>AAEKGFKQAFWQPLCQVSEELDDQPKGALFTLQAAASKIQKMRD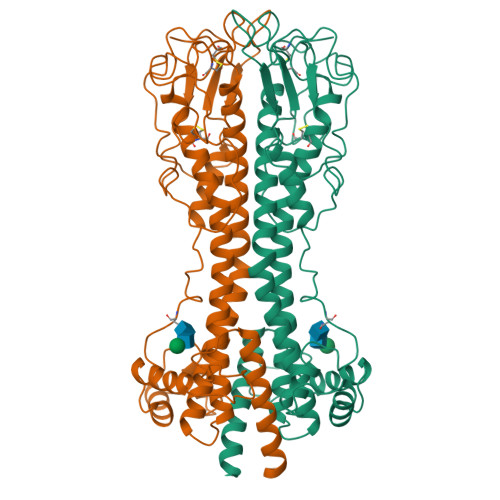AALRASIYAEINHGTNRAKAAVIVANHYAMKADSGLEALKQTLSSQEVTATATASYLKGRIDEYLNLLLQTKESGTSGCMMDTSGTNTVTKAGGTIGGVPCKLQLSPIQPKRPAATYLGKAGYVGLTRQADAANNFHDNDAECRLASGHNTNGLGKSGQLSAAVTMAAGYVTVANSQTAVTVQALDALQEASGAAHQPWIDAWKAKKALTGAETAEFRNETAGIAGKTGVTKLVEEALLKKKDSEASEIQTELKKYFSGHENEQWTAIEKLISEQPVAQNLVGDNQPTKLGELEGNAKLTTILAYYRMETAGKFEVLTQK[2x]>[6x]MRRRSRMLLCFAFLWVLGIAYYMYSGGGSALAGGAGGGAGRKEDWNEIDPIKKKDLHHSNGEEKAQSMETLPPGKVRWPDFNQEAYVGGTMVRSGQDPYARNKFNQVESDKLRMDRAIPDTRHDQCQRKQWRVDLPATSVVITFHNEARSALLRTVVSVLKKSPPHLIK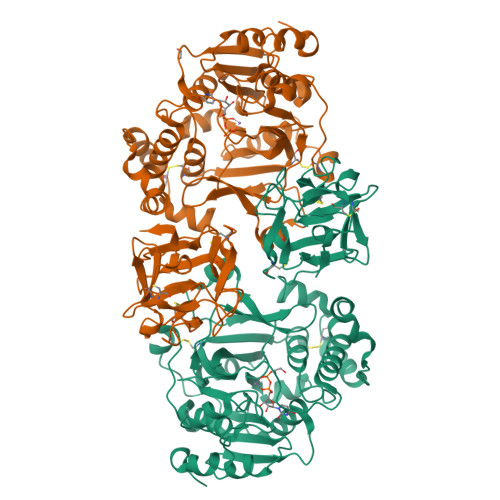EIILVDDYSNDPEDGALLGKIEKVRVLRNDRREGLMRSRVRGADAAQAKVLTFLDSHCECNEHWLEPLLERVAEDRTRVVSPIIDVINMDNFQYVGASADLKGGFDWNLVFKWDYMTPEQRRSRQGNPVAPIKTPMIAGGLFVMDKFYFEELGKYDMMMDVWGGENLEISFRVWQCGGSLEIIPCSRVGHVFRKQHPYTFPGGSGTVFARNTRRAAEVWMDEYKNFYYAAVPSARNVPYGNIQSRLELRKKLSCKPFKWYLENVYPELRVPDHQDIAFGALQQGTNCLDTLGHFADGVVGVYECHNAGGNQEWALTKEKSVKHMDLCLTVVDRAPGSLIKLQGCREDDSRQKWEQIEGNSKLRHVGSNLCLDSRTAKSGGLSVEVCGPALSQQWKFTLNLQQ5-chloro-N-[1-(2-{[2-fluoro-4-(2-oxopyridin-1(2H)-yl)phenyl]amino}-2-oxoethyl)-1H-1,2,4-triazol-3-yl]thiophene-2-carboxamide 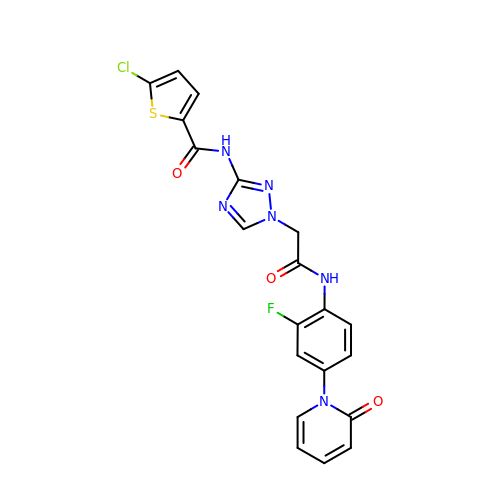| C20 H14 Cl F N6 O3 S | KAUVVMPQUJSRIS-UHFFFAOYSA-N> QAQITGRPEWIWLALGTALMGLGTLYFLVKGMGVSDPDAKKFYAITTLVPAIAFTMYLSMLLG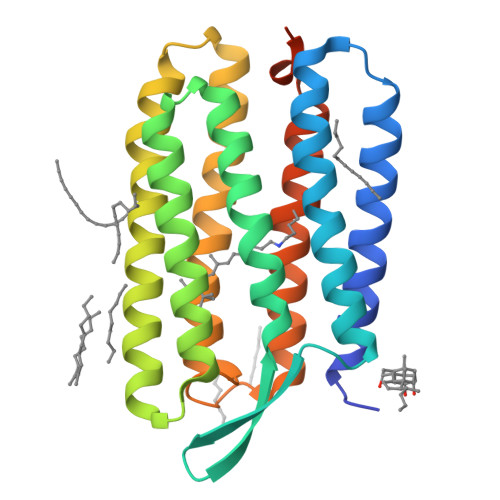YGLTMVPFGGEQNPIYWARYADWLFTTPLLLLDLALLVDADQGTILALVGADGIMIGTGLVGALTKVYSYRFVWWAISTAAMLYALYVLFFGFTSKAESMRPEVASTFKVLRNVTVVLWSAYPVVWLIGSEGAGIVPLNIETLLFMVLDVSAKVGFGLILLRSRAIFGEAEAPEPSAGDGAAATSD2-pyridin-3-yl-1,3-benzothiazin-4-one 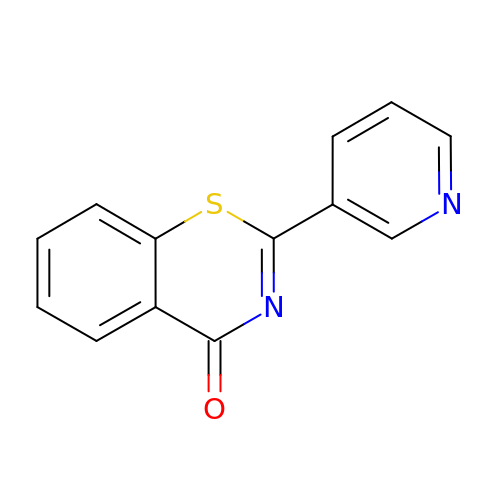| C13 H8 N2 O S | PKPRJBMZCMHZGS-UHFFFAOYSA-N>SNAMHILVTGFAPFDNQNINPSWEAVTQLEDIIGTHTIDKLKLPTSFKKVDNIINKTLASNHYDVVLAIGQAGGRNAITPERVAINIDDARIPDNDDFQPIDQAIHLDGAPAYFSNLPVKAMTQSIINQGLPGALSNSAGTFVCNH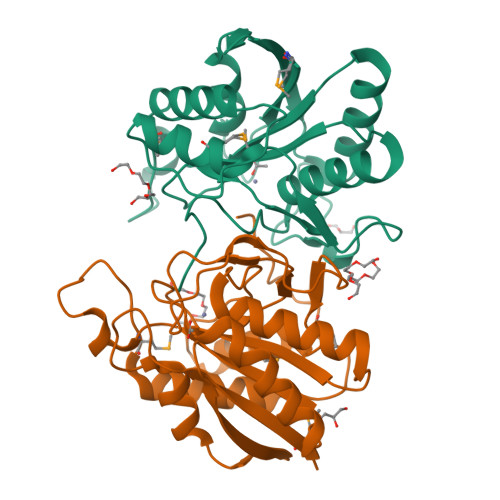TLYHLGYLQDKHYPHLRFGFIHVPYIPEQVIGKPDTPSMPLEKIVAGLTAAIEAISNDEDLHLALGTTE[2x]> IESIIKTATDTVKSEINAELGVVPSLNAVETGATSNTEPEEAIQTRTVINQHGVSETLVENFLSRAALVSKRSFEYKDHTSSTARADKNFFKWTINTRSFVQLRRKLELFTYLRFD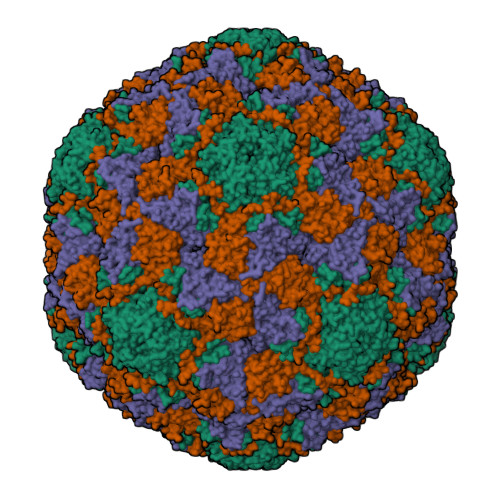AEITILTTVAVNGSGNNTYVGLPDLTLQAMFVPTGALTPEKQDSFHWQSGSNASVFFKISDPPARITIPFMCINSAYSVFYDGFAGFEKNGLYGINPADTIGNLCVRIVNEHQPVGFTVTVRVYMKPKHIKAWAPRPPRTLPYMSIANANYKGKERAPNALSAIIGNRDSVKTMPHNIVNT;> GVPTYLLPGSGQFLTTDDHSSAPALPCFNPTPEMHIPGQVRNMLEVVQVESMMEINNTESAVGMERLKVDISALTDVDQLLFNIPLDIQLDGPLRNTLVGNISRYYTHWSGSLEMTFMFCGSFMAAGKLILCYTPPGGSCPTTRETAMLGTHIVWDFGLQSSVTLIIPWISGSHYRMFNNDAKSTNANVGYVTCFMQTNLIVPSESSDTCSLIGFIAAKDDFSLRLMRDSPDIGQLDHLHAAEAAYQ;> SPSAEACGYSDRVLQLKLGNSAIVTQEAANYCCAYGEWPNYLPDHEAVAIDKPTQPETATDRFYTLKSVKWETGSTGWWWKLPDALNNIGMFGQNVQHHYLYRSGFLIHVQCNATKFHQGALLVVAIPEHQRGAHNTNTSPGFDDIMKGEEGGTFNHPYVLDDGTSLACATIFPHQWINLRTNNSATIVLPWMNAAPMDFPLRHNQWTLAIIPVVPLGTRTTSSMVPITVSIAPMCCEFNGLRHAITQ> GYEEREGGFRKETVER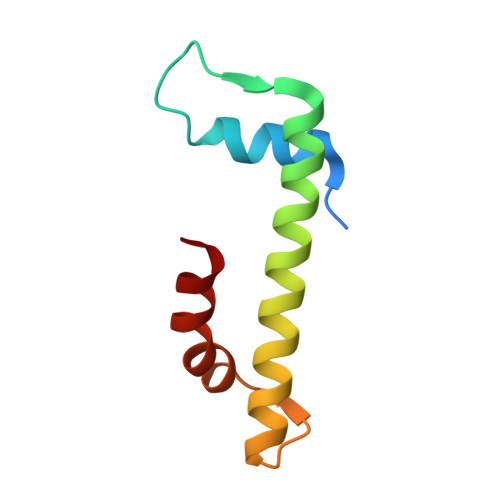LLRLHFRDGRTRVNGDALLLMAELLKVFVREAAARAARQAQAEDLEKVDIEHVEKVLPQLLLDFV>HHHHHHSSGLVPRGSMDIRALYDEKLTTPEEAVSSIASGSHLSMGMFAAEPPALLKALADRATRGDIGDLRVYYFETAKIAGDTILRYELNNRIKPYSMFVTAVERALIRRGIEDGGRKVVNYVPSNFHQAPRLLAEEIGIDTFMHTVSPMDCHGYFSLGVGNDYSSRIARSARRFIVEVNRYMPRVQGEAAAIHISEVDAIVENHVPLIEMPVRSAIPEYTSISHIIADLVPDGACLQMGVGALPNLVCGVLKDRNDLGIHTEVLNPGLVDLIRRGVVTNQRKTLDRGRSVFTFAMGQQEMYEYLNDHPAIFSRPVDYVNDPHIIAQNDNVVSINATLQIDLTGACNSEHMLGHQYSASGGQLDFVRGAYASKGGRSIIATPSTAAKGTVSRIIPRIDGPVTTPRIDTHYIVTEFGAVNLKGLSSTERALRIIELAHPDFRDELTQAAKKMHLI[2x]

Thus, ripA and ripB along with a third gene ripC, constitute a novel virulence operon designated rip (required for intracellular proliferation), thought to be important in intracellular replication of Y. pestis in macrophages. The ripA gene encodes for a protein highly homologous to 4-hydroxybutyrate-CoA transferase (4-HB-CoAT), which belongs to a superfamily of CoA transferases responsible for the transfer of the CoAS− anion from a donor CoA thioester to an acceptor free acid. Further, CoA transferase activity assays suggest that RipA has a preference for butyryl or propionyl moieties compared to 4-hydroxybutyryl. Herein, we suggest that in INF-g activated macrophages, RipA, a proposed butyryl-CoA transferase, produces butyrate that indirectly lowers the macrophage NO levels, preventing bacterial cell death.

Additionally, we report the 1.9 Å crystal structure of tetrameric RipA and demonstrate that this oligomeric state is stable in solution suggesting that the physiologically relevant assembly of RipA is tetrameric. Two homodimers form a doughnut-like tetramer where the buried surface area between each monomer at the dimer-dimer interface of the tetramer is 1454 Å2 (calculated with AreaiMol), which is ∼8.2% of the total surface area. The dimer-dimer interface is facilitated by weak interactions between residues from both domains. Although a network of ordered dimer-dimer interface waters facilitates tetramer formation in both RipA and YdiF, the increased buried surface and direct residue contacts found in RipA likely results in a more stable tetramer. As there are no existing butyryl-CoA transferase structures, the 1.9 Å RipA crystal structure, which demonstrates the canonical Family I CoA transferases α/β fold, is compared against 4-HB-CoAT structures. The overall fold amongst the RipA and 4-HB-CoAT structures are highly conserved with RMSDs between 1.57–1.68 Å in pairwise structural alignments. The RipA structure most likely represents a form similar to the unbound form crystallized with glycerol, as RipA was also crystallized with glycerol. With the exception of Glu61, which is protonated and polar, the pocket is entirely apolar, resembling those described in C. aminobutyricum 4-HBCoAT and SCOT with Phe85, Phe60 and Phe113 conserved in all 4-HBCoATs. The pocket size, which restricts the size of the acyl group that can bind effectively, appears to be large enough to accommodate acyl groups of three to four carbon atoms and helps explain the competition and DSF assays.> SNATDSTVSTDPVTLNTEKTTLDQDVVINGDNKITAVTIETSDSDKDLNVTFGGHDITATSTVNQDFVEGVKVSGNKNVVINATDSTITAQGEGTYVRTAMVIDSTGDVVVNGGNFVAKNEKGSATGISLEATTGNNLTLNGTTINAQGNKSYSNGSTAIFAQKGNLLQGFDGDATDNITLADSNIINGGIETIVTAGNKTGIHTVNLNIKDGSVIGAANNKQTIYASASAQGAGSATQNLNLSVADSTIYSDVLALSESENSASTTTNVNMN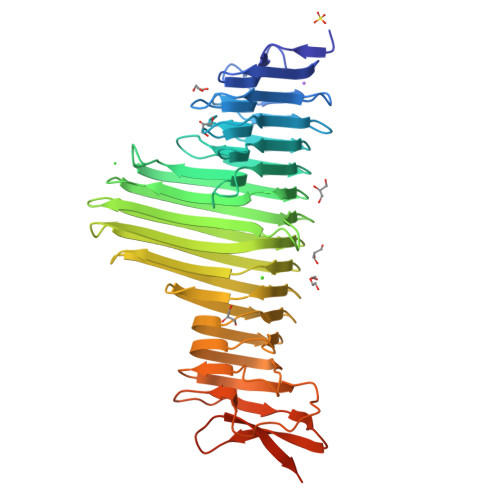VARSYWEGNAYTFNSGDKAGSDLDINLSDSSVWKGKVSGAGDASVSLQNGSVWNVTGSSTVDALAVKDSTVNITKATVNTGTFASQNGTLIVDASSENTLDISGKASGDLRVYSAGSLDLINEQTAFISTGKDSTLKATGTTEGGLYQYDLTQGADGNFYFVKNTHKASNASSVIQAMAAAPANVANLQADTL CaNMT shares 44% and 43% sequence identity with P. vivax and L. donovani NMTs (PvNMT, LdNMT) respectively; we reasoned that inhibitors of Plasmodium and Leishmania NMTs might be acquired through a ‘piggy-back’ approach, using CaNMT peptidomimetics as a platform. We therefore chose to employ a similar peptidomimetic scaffold based on the Ser-Lys motif, substituting the first four amino acids with an alkyl chain capped by a group that mimics the N-terminal amine, and the C-terminal leucine with a hydrophobic motif. The N-terminal motif of the peptidomimetic was expected to interact directly with the C-terminal carboxylate leucine of the enzyme, a critical residue for catalytic activity responsible for the activation of the N-terminal amine of the protein/peptide substrate. Using antifungal NMT inhibitors as a platform, we developed inhibitors of Plasmodium and Leishmania NMTs, resulting in the identification of an inhibitor, 10, with sub-micromolar potency against P. vivax and L. donovani NMTs, and the most potent Leishmania donovani NMT inhibitor reported to date.

Reduction of the alkyl chain length from n = 10 to 9 gave compound 10, which is the most potent L. donovani NMT inhibitor reported to date (LdNMT IC50 = 24 nM). It also showed somewhat lower activity against HsNMT1 (IC50 = 60 nM) and PvNMT (680 nM). High-resolution ternary structures of compound 10 were achieved in both PvNMT and LmNMT, with the latter structure revealing the first structural evidence supporting the proposed catalytic cycle of NMT. 10 sits in the peptide-binding pocket, and mimics the key recognition elements involved in binding the parent peptide (GLYASKL). The N-terminal amine electrostatically interacts with the carboxylate of Leu410 whilst the hydroxyl group of the serine hydrogen bonds to the His213 side chain. In addition, there are ionic interactions between the amino group of the lysine and three neighboring aspartic acid residues (Asp98, Asp100, Asp385), all of which are conserved in equivalent residues CaNMT. The aliphatic chain on the N-terminus and the N-terminal amino group of the inhibitor are guided by the peptide binding channel to the C-terminal residue of PvNMT–Leu410. Unusually, the inhibitors in this study showed a higher specificity for P. vivax NMT in comparison to P. falciparum NMT. An alignment of the primary sequences of both enzymes (see ESI†) highlighted four differing residues within 6 Å of the peptide binding pocket: Ile102, Tyr212, Ser228, Tyr334 (PvNMT) and Val102, Phe212, Cys228 and Phe334 (PfNMT). Of these differences, the replacement of Y334 to F334 in PfNMT constitutes a structural change in the peptide pocket that could lead to a loss of potential hydrogen bond interactions within the catalytic site.

>DYKFWYTQPVPKINDEFNESVNEPFISDNKVEDVRKDEYKLPPGYSWYVCDVKDEKDRSEIYTLLTDNYVEDDDNIFRFNYSAEFLLWALTSPNYLKTWHIGVKYDASNKLIGFISAIPTDICIHKRTIKMAEVNFLCVHKTLRSKRLAPVLIKEITRRINLENIWQAIYTAGVYLPKPVSDARYYHRSINVKKLIEIGFSSLNSRLTMSRAIKLYRVEDTLNIKNMRLMKKKDVEGVHKLLGSYLEQFNLYAVFTKEEIAHWFLPIENVIYTYVNEENGKIKDMISFYSLPSQILGNDKYSTLNAAYSFYNVTTTATFKQLMQDAILLAKRNNFDVFNALEVMQNKSVFEDLKFGEGDGSLKYYLYNWKCASFAPAHVGIVLL[3x]>[2x]TRLGLEDFESLKVIGR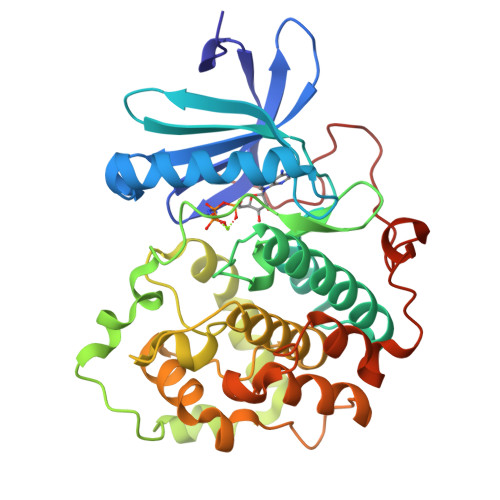GAFGEVRLVQKKDTGHVYAMKILRKADMLEKEQVGHIRAERDILVEADSLWVVKMFYSFQDKLNLYLIMEFLPGGDMMTLLMKKDTLTEEETQFYIAETVLAIDSIHQLGFIHRDIKPDNLLLDSKGHVKLSDFGLCTGLKKAHRTEFYRNLNHSLPSDFTFQNMNSKRKAETWKRNRRQLAFSTVGTPDYIAPEVFMQTGYNKLCDWWSLGVIMYEMLIGYPPFCSETPQETYKKVMNWKETLTFPPEVPISEKAKDLILRFCCEWEHRIGAPGVEEIKSNSFFEGVDWEHIRERPAAISIEIKSIDDTSNFDEFP methyl 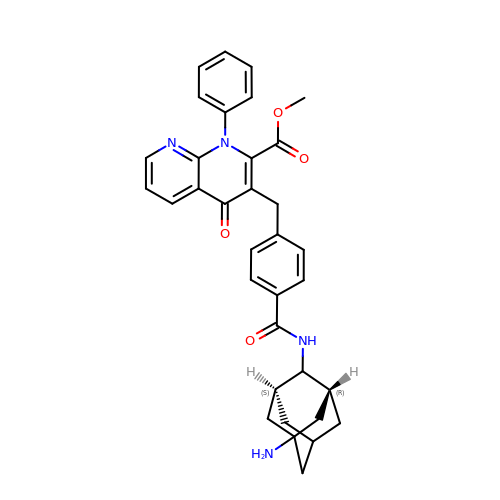3-(4-{[(1R,2S,3S,5S,7s)-5-aminotricyclo[3.3.1.1~3,7~]dec-2-yl]carbamoyl}benzyl)-4-oxo-1-phenyl-1,4-dihydro-1,8-naphthyridine-2-carboxylate | C34 H34 N4 O4 | OVPCOPWFTZDTCI-CJYKQNLHSA-N> MGHHHHHHHHHHSSGHIEGRHMLRERTVRLQYGSRVEAVYVLGTYLWTDVYSAAPAGAQTFSLKHSEHVWVEVVRDGEAEEVATNGKQRWLLSPSTTLRVTMSQASTEASSDKVTVNYYDEEGSIPIDQAGLFLTAIEISLDVNADRDGVVEKNNPKKASWTWGPEGQGAILLVNCDRETPWLPKEDCRDEKVYSKEDLKDMSQMILRTKGPDRLPAGYEIVLYISMSDSDKVGVFYVENPFFGQRYIHILGRRKLYHVVKYTGGSAELLFFVEGLCFPDEGFSGLVSIHVSLLEYMAQDIPLTPIFTDTVIFRIAPWIMTPNILPPVSVFVCCMKDNYLFLKEVKNLVEKTNCELKVCFQYLNRGDRWIQDEIEFGYIEAPHKGFPVVLDSPRDGNLKDFPVKELLGPDFGYVTREPLFESVTSLDSFGNLEVSPPVTVNGKTYPLGRILIGSSFPLSGGRRMTKVVRDFLKAQQVQAPVELYSDWLTVGHVDEFMSFVPIPGTKKFLLLMASTSACYKLFREKQKDGHGEAIMFKGLGGMSSKRITINKILSN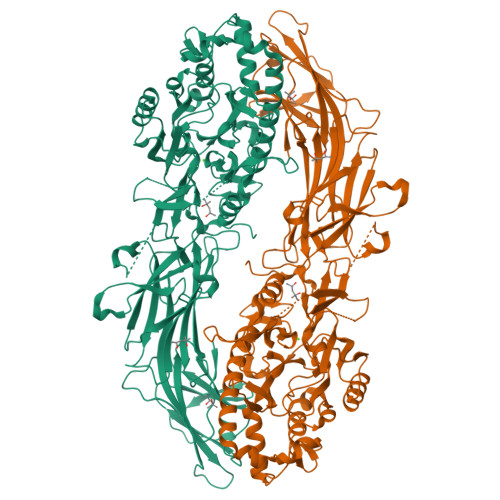ESLVQENLYFQRCLDWNRDILKKELGLTEQDIIDLPALFKMDEDHRARAFFPNMVNMIVLDKDLGIPKPFGPQVEEECCLEMHVRGLLEPLGLECTFIDDISAYHKFLGEVHCGTNVRRKPFTFKWWHMVPSRRS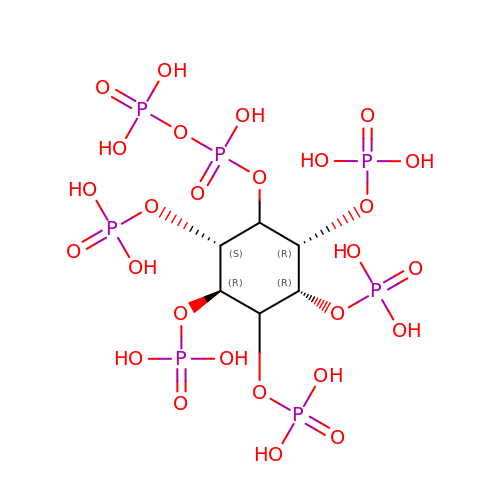(1R,2R,3R,4R,5R,6S)-2,3,4,5,6-pentakis(phosphonooxy)cyclohexyl trihydrogen diphosphate | C6 H19 O27 P7 | UPHPWXPNZIOZJL-XCMZKKERSA-N PIEZO channels transmit mechanical force signals to cells, allowing them to make critical decisions during development and in pathophysiological conditions. Here, we report several near-atomic resolution cryo-EM structures of fast-inactivating wild-type human PIEZO1 (hPIEZO1) and its slow-inactivating channelopathy mutants with or without its auxiliary subunit MDFIC. Each hPIEZO1 subunit has a curved blade structure, and the three subunits form the trimeric PIEZO channel, exhibiting a bowl-like shape. MDFIC, a MyoD family inhibitor protein, has recently been identified as an auxiliary subunit of piezo channels capable of decelerating channel inactivation and attenuating channel mechanosensitivity.

The multi-lipidated MDFIC subunits insert laterally into the hPIEZO1 pore module like mPIEZO1, resulting in a more curved and extended state. To solve the structural basis of MDFIC on hPIEZO1, we co-expressed it with hMDFIC in HEK293F and purified the complex. We obtained a 3.0 Å resolution cryo-EM density map of the hPIEZO1-MDFIC complex. The overall cryo-EM density map is similar to hPIEZO1 alone with a disk of about 30 nm, but allowed us to validate the MDFIC density with multi-lipidated cysteines on the C-terminal amphipathic helix. This C-terminal helix inserted laterally into the pore module where the exact position of mPIEZO1 is found. Interestingly, while MDFIC does not significantly alter the curvature of mPIEZO1, it induces a more curved and contracted architecture in hPIEZO1 from the side and top views, respectively. Combining with the similar effect of MDFIC on mPIEZO1 and hPIEZO1, we suspect that MDFIC decelerates hPIEZO1 inactivation and weakens its mechanosensitivity by remodeling the pore module and exerting more blade curvature. We were surprised to find an apparent lipid density in wild-type hPIEZO1-MDFIC, hPIEZO1-A1988V-MDFIC, and even more evident in the 2.8 Å resolution map of hPIEZO1-E756del-MDFIC in the pore module, where one of its hydrophobic fatty acid tails inserts into the hydrophobic pore formed by I2447, V2450, and F2454, thus sealing the pore to prevent ion flow. In addition, another fatty acid chain of the pore lipid interacts with the acyl chains of the covalently linked MDFIC lipids, forming a stable hPIEZO1-multi-lipidated MDFIC-pore lipid complex. Therefore, we deduce that the hPIEZO1-MDFIC/hPIEZO1-A1988V-MDFIC/hPIEZO1-E756del-MDFIC reshape the pore module and fall into a deep resting state, in which it becomes rather tricky to remove the pore lipid from the hydrophobic pore by mild mechanical force.

>[3x]MEPHVLGAVLYWLLLPCALLAACLLRFSGLSLVYLLFLLLLPWFPGPTRCGLQGHTGRLLRALLGLSLLFLVAHLALQICLHIVPRLDQLLGPSCSRWETLSRHIGVTRLDLKDIPNAIRLVAPDLGILVVSSVCLGICGRLARNTRQSPHPRELDDDERDVDASPTAGLQEAATLAPTRRSRLAARFRVTAHWLLVAAGRVLAVTLLALAGIAHPSALSSVYLLLFLALCTWWACHFPISTRGFSRLCVAVGCFGAGHLICLYCYQMPLAQALLPPAGIWARVLGLKDFVGPTNCSSPHALVLNTGLDWPVYASPGVLLLLCYATASLRKLRAYRPSGQRKEAAKGYEARELELAELDQWPQERESDQHVVPTAPDTEADNCIVHELTGQSSVLRRPVRPKRAEPREASPLHSLGHLIMDQSYVCALIAMMVWSITYHSWLTFVLLLWACLIWTVRSRHQLAMLCSPCILLYGMTLCCLRYVWAMDLRPELPTTLGPVSLRQLGLEHTRYPCLDLGAMLLYTLTFWLLLRQFVKEKLLKWAESPAALTEVTVADTEPTRTQTLLQSLGELVKGVYAKYWIYVCAGMFIVVSFAGRLVVYKIVYMFLFLLCLTLFQVYYSLWRKLLKAFWWLVVAYTMLVLIAVYTFQFQDFPAYWRNLTGFTDEQLGDLGLEQFSVSELFSSILVPGFFLLACILQLHYFHRPFMQLTDMEHVSLPGTRLPRWAHRQDAVSGTPLLREEQQEHQQQQQEEEEEEEDSRDEGLGVATPHQATQVPEGAAKWGLVAERLLELAAGFSDVLSRVQVFLRRLLELHVFKLVALYTVWVALKEVSVMNLLLVVLWAFALPYPRFRPMASCLSTVWTCVIIVCKMLYQLKVVNPQEYSSNCTEPFPNSTNLLPTEISQSLLYRGPVDPANWFGVRKGFPNLGYIQNHLQVLLLLVFEAIVYRRQEHYRRQHQLAPLPAQAVFASGTRQQLDQDLLGCLKYFINFFFYKFGLEICFLMAVNVIGQRMNFLVTLHGCWLVAILTRRHRQAIARLWPNYCLFLALFLLYQYLLCLGMPPALCIDYPWRWSRAVPMNSALIKWLYLPDFFRAPNSTNLISDFLLLLCASQQWQVFSAERTEEWQRMAGVNTDRLEPLRGEPNPVPNFIHCRSYLDMLKVAVFRYLFWLVLVVVFVTGATRISIFGLGYLLACFYLLLFGTALLQRDTRARLVLWDCLILYNVTVIISKNMLSLLACVFVEQMQTGFCWVIQLFSLVCTVKGYYDPKEMMDRDQDCLLPVEEAGIIWDSVCFFFLLLQRRVFLSHYYLHVRADLQATALLASRGFALYNAANLKSIDFHRRIEEKSLAQLKRQMERIRAKQEKHRQGRVDRSRPQDTLGPKDPGLEPGPDSPGGSSPPRRQWWRPWLDHATVIHSGDYFLFESDSEEEEEAVPEDPRPSAQSAFQLAYQAWVTNAQAVLRRRQQEQEQARQEQAGQLPTGGGPSQEVEPAEGPEEAAAGRSHVVQRVLSTAQFLWMLGQALVDELTRWLQEFTRHHGTMSDVLRAERYLLTQELLQGGEVHRGVLDQLYTSQAEATLPGPTEAPNAPSTVSSGLGAEEPLSSMTDDMGSPLSTGYHTRSGSEEAVTDPGEREAGASLYQGLMRTASELLLDRRLRIPELEEAELFAEGQGRALRLLRAVYQCVAAHSELLCYFIIILNHMVTASAGSLVLPVLVFLWAMLSIPRPSKRFWMTAIVFTEIAVVVKYLFQFGFFPWNSHVVLRRYENKPYFPPRILGLEKTDGYIKYDLVQLMALFFHRSQLLCYGLWDHEEDSPSKEHDKSGEEEQGAEEGPGVPAATTEDHIQVEARVGPTDGTPEPQVELRPRDTRRISLRFRRRKKEGPARKGAAAIEAEDREEEEGEEEKEAPTGREKRPSRSGGRVRAAGRRLQGFCLSLAQGTYRPLRRFFHDILHTKYRAATDVYALMFLADVVDFIIIIFGFWAFGKHSAATDITSSLSDDQVPEAFLVMLLIQFSTMVVDRALYLRKTVLGKLAFQVALVLAIHLWMFFILPAVTERMFNQNVVAQLWYFVKCIYFALSAYQIRCGYPTRILGNFLTKKYNHLNLFLFQGFRLVPFLVELRAVMDWVWTDTTLSLSSWMCVEDIYANIFIIKCSRETEKKYPQPKGQKKKKIVKYGMGGLIILFLIAIIWFPLLFMSLVRSVVGVVNQPIDVTVTLKLGGYEPLFTMSAQQPSIIPFTAQAYEELSRQFDPQPLAMQFISQYSPEDIVTAQIEGSSGALWRISPPSRAQMKRELYNGTADITLRFTWNFQRDLAKGGTVEYANEKHMLALAPNSTARRQLASLLEGTSDQSVVIPNLFPKYIRAPNGPEANPVKQLQPNEEADYLGVRIQLRREQGAGATGFLEWWVIELQECRTDCNLLPMVIFSDKVSPPSLGFLAGYGIMGLYVSIVLVIGKFVRGFFSEISHSIMFEELPCVDRILKLCQDIFLVRETRELELEEELYAKLIFLYRSPETMIKWTREKE;>[3x]MSGAGEALAPGPVGPQRVAEAGGGQLGSTAQGKCDKDNTEKDITQATNSHFTHGEMQDQSIWGNPSDGELIRTQPQRLPQLQTSAQVPSGEEIGKIKNGHTGLSNGNGIHHGAKHGSADNRKLSAPVSQKMHRKIQSSLSVNSDISKKSKVNAVFSQKTGSSPEDCCVHCILACLFCEFLTLCNIVLGQASCGICTSEACCCCCGDEMGDDCNCPCDMDCGIMDACCESSDCLEICMECCGICFPS> VVVEDSGASFGESLLDTTSEPGK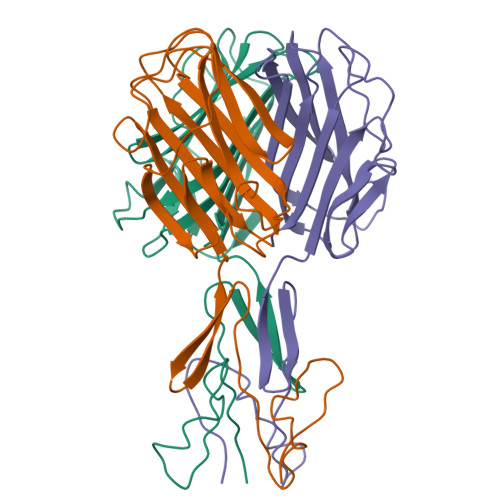ILVKRISGGSGITVTDYGDQVEIEASVTDALSLMYSTSTGGPASIAANALTDFDLSGALTVNSVGTGLTKSAAGIQLAAGKSGLYQITMTVKNNTVTTGNYLLRVKYGSSDFVVACPASSLTAGGTISLLIYCNVLGVVSLDVLKFSLCNDGAALSNYIINITAAKIN> MGKNLSLRQDDAQHALSANTSSAYNSVYDFLRYHDRGDGLTVNGKTSYSIDQAAAQITRENVSWNGTNVFGKSANLTFKFLQSVSSIPSGDTGFVKFNAEQIEQAKLSLQSWSDVANLTFTEVTGNKSANITFGNYTRDASGNLDYGTQAYAY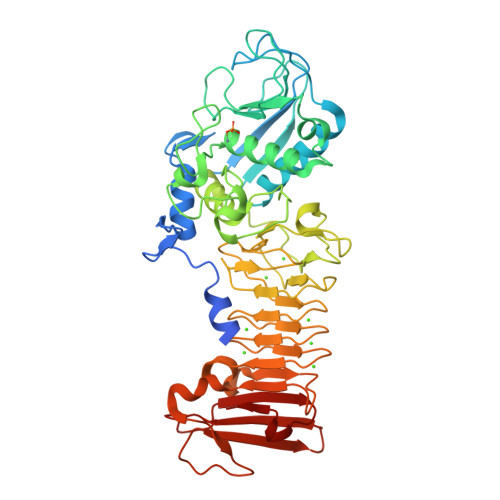YPGNYQGAGSSWYNYNQSNIRNPGSEEYGRQTFTHEIGHALGLAHPGEYNAGEGDPSYNDAVYAEDSYQFSIMSYWGENETGADYNGHYGGAPMIDDIAAIQRLYGANMTTRTGDSVYGFNSNTDRDFYTATDSSKALIFSVWDAGGTDTFDFSGYSNNQRINLNEGSFSDVGGLKGNVSIAHGVTIENAIGGSGNDILVGNSADNILQGGAGNDVLYGGAGADTLYGGAGRDTFVYGSGQDSTVAAYDWIADFQKGIDKIDLSAFRNEGQLSFVQDQFTGKGQEVMLQWDAANSITNLWLHEAGHSSVDFLVRIVGQAAQSDIIV>[2x]XAAAALAA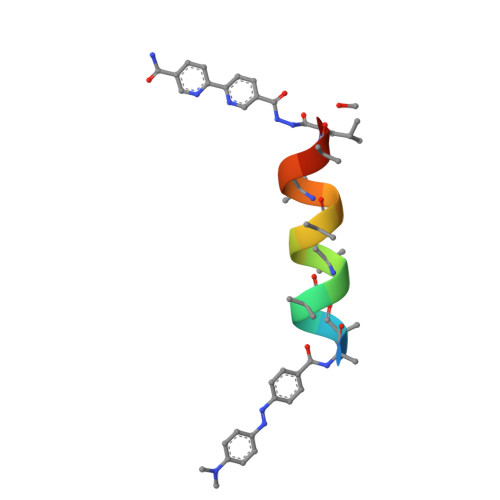ALAQALX>GADILNCILPAEMLTGTDIDYNRPYDKSLNAYPIYIEVNNGTDLTRLAPTFELTEGASIEPANGSTQNFTNPVRYTVTSEDKNWHRTYAINIHYPETKSIPTVFNFENVKTVPYNKNEYYVLYEAASGYSTLTWSSGNQGFALTGSGYTPNDFPTSISPNGRTGNCLQLITRKTGSLGTLVGMPIAAGNLFIGSFDIGSAMSDALSATKFGTTFYYEPI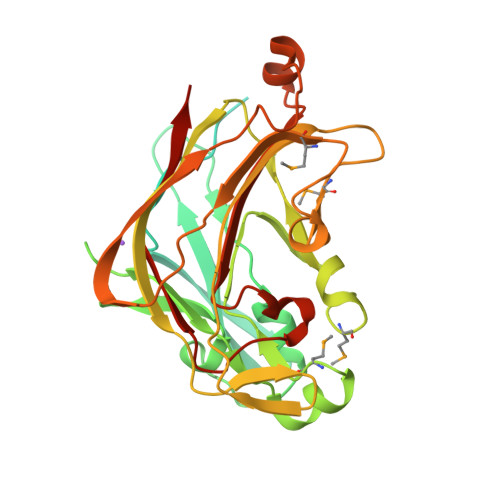KLVGYYKYKAGPEFYENGESTNRKDVFNIYALFYEKTKDVQMLDGHIAKNNYEHENMVAAAVITDTHETSEWTRFELDFNYEHYGKTIDPQKLANGGYNVSIVLSASKDGDVFQGAPGSTLLIDDLELVCKQPLR[2x]> MGERPPPKRLTREAMRNYLKERGDQTVLILHAKVAQKSYGNEKRFFCPPPCVYLMGSGWKKKKEQMERDGCSEQESQPCAFIGIGNSDQEMQQLNLEGKNYCTAKTLYISDSDKRKHFMLSVKMFYGNSDDIGVFLSKRIKVISKPSKKKQSLKNADLCIASGTKVALFNRLRSQTVSTRYLHVEGGNFHASSQQWGAFFIHLLDDDESEGEEFTVRDGYIHYGQTVKLVCSVTGMALPRLIIRKVDKQTALLDADDPVSQLHKCAFYLKDTERMYLCLSQERIIQFQATPCPKEPNKEMINDGASWTIISTDKAEYTFYEGMGPVLAPVTPVPVVESLQLNGGGDVAMLELTGQNFTPNLRVWFGDVEAETMYRCGESMLCVVPDISAFREGWRWVRQPVQVPVTLVRNDGIIYSTSLTFTYTPEPGHHHHHH;> GMDVNVRGPDGFTPLMIASCSGGGLETGNSEEEEDAPAVISDFIYQGASLHNQTDRTGETALHLAARYSRSDAAKRLLEASADANIQDNMGRTPLHAAVSADAQGVFQILIRNRATDLDARMHDGTTPLILAARLAVEGMLEDLINSHADVNAVDDLGKSALHWAAAVNNVDAAVVLLKNGANKDMQNNREETPLFLAAREGSYETAKVLLDHFANRDITDHMDRLPRDIAQERMHHDIVRLLDEYNLVRSPQLHG;> GLPRHSAVMERLRRRIELCRRHHSTCEARYEAVSPERLELERQHTFALHQRCIQAKAKRAGKH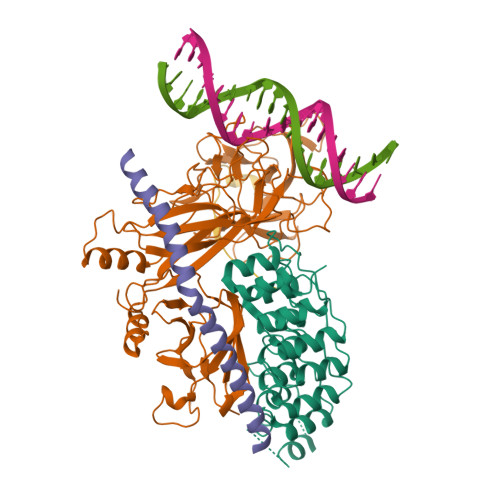;> KRRRQHGQLWFPEGFKVSE>SSNDNIELVDFQNIMFYGDAEVGDNQQPFTFILDTGSANLWVPSVKCTTAGCLTKHLYDSSKSRTYEKDGTKVEMNYVSGTVSGFFSKDLVTVGNLSLPYKFIEVIDTNGFEPTYTASTFDGILGLGWKDLSIGSVDPIVVELKNQNKIENALFTFYLPVHDKHTGFLTIGGIEERFYEGPLTYEKLNHDLYWQITLDAHVGNISLEKANCIVDSGTSAITVPTDFLNKMLQNLDVIKVPFLPFYVTLCNNSKLPTFEFTSE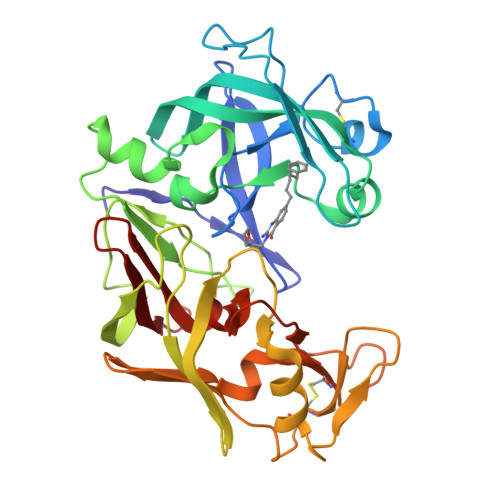NGKYTLEPEYYLQHIEDVGPGLCMLNIIGLDFPVPTFILGDPFMRKYFTVFDYDNHSVGIALAKKNL[4x]>[3x]MANPLYQKHIISINDLSRDDLNLVLATAAKLKANPQPEL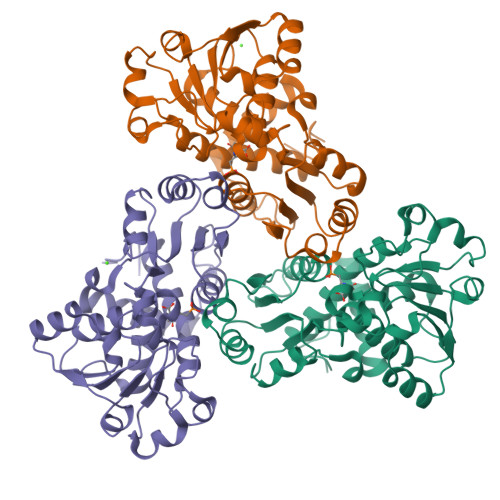LKHKVIASCFFEASTRTRLSFETSMHRLGASVVGFSDSANTSLGKKGETLADTISVISTYVDAIVMRHPQEGAARLATEFSGNVPVLNAGDGSNQHPTQTLLDLFTIQETQGRLDNLHVAMVGDLKYGRTVHSLTQALAKFDGNRFYFIAPDALAMPQYILDMLDEKGIAWSLHSSIEEVMAEVDILYMTRVQKERLDPSEYANVKAQFVLRASDLHNAKANMKVLHPLPRVDEIATDVDKTPHAWYFQQAGNGIFARQALLALVLNRDLVL> MILIGDSGSTKTDWCIAKEGKSLGRFQTSGINPFQQDRNEIDTALRSEVLPAIGQKASSIRAVYFYGAGCTPAKAPMLNEALDSMLPHCDRIEVAGDMLGAARALCGDSEGIACILGT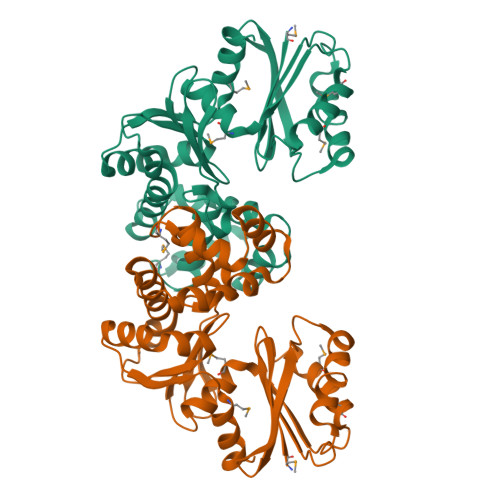GSNSCLFDGREIKANVSPLGYILGDEGSGAVLGRLFIGSLLKGQMPEGLCEAFLQEYGLTSADIIESVYRKPFPNRFLAGFSPFIAQHLDIPAVYSLVQNSFDDFLVRNVLRYNRPDLPLHFIGSVAFHYREVLSSVIKKRGLTLGSVLQSPMEGLIQYHHNNHVLEHHHHHH> GHMSPNYDKWEMERTDITMKHKLGGGQYGEVYEGVWKKYSLTVAVKTLKEDTMEVEEFLKEAAVMKEIKHPNLVQLLGVCTREPPFYIITEFMTYGNLLDYLRECNRQEVNAVVLLYMATQISSAMEYLEKKNFIHRDLAARNCLVGENHLVKVADFGLSRLMTGDTYTAHAGAKFPIKWTAPESLAYNKFSIKSDVWAFGVLLWEIATYGMSPYPGIDLSQVYELLEKD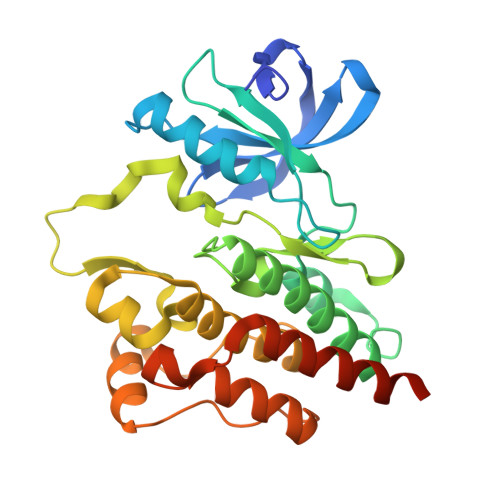YRMERPEGCPEKVYELMRACWQWNPSDRPSFAEIHQAFETMFQESSISDEVEKELGK Pinoresinol/lariciresinol reductase (PLR), an NADPH-dependent reductase, converts pinoresinol to lariciresinol and subsequently to secoisolariciresinol. Here, we present crystal structures of IiPLR1 from Isatis indigotica and pinoresinol reductases (PrRs) AtPrR1 and AtPrR2 from Arabidopsis thaliana, in the apo, substrate-bound and product-bound states. The crystal structures were captured in the apo, substrate-bound and/or product-bound forms. We found that, for all 16 structures we solved, each enzyme adopts a similar head-to-tail dimer conformation, strongly suggesting that each PLR/PrR functions as a homodimer, consistent with the literature that TpPLR1 exists as a dimeric entity in solution. Each structure contains a head-to-tail homodimer, and the catalytic pocket comprises structural elements from both monomers. β4 loop covers the top of the pocket, and residue 98 from the loop governs catalytic specificity.

Known exceptions are Arabidopsis thaliana reductases that have substrate preference for pinoresinol, but only weak (AtPrR1) or no activity (AtPrR2) toward lariciresinol and are thus named pinoresinol reductases (PrRs). Each of IiPLR1_NAP_ + PIN/AtPrR1_NAP_ + PIN/AtPrR2_NAP_ + PIN forms a homodimer, and superimposition of the protomers among the three complexes revealed RMSDs of 0.374, 0.365, and 0.308 Å, respectively. In contrast to IiPLR1_NAP_ + PIN, the β4 loops of AtPrR1_NAP_ + PIN and AtPrR2_NAP_ + PIN can be clearly identified. These well-defined loops twist as an “8” shape and cover both the NADP+-binding and substrate-binding grooves. Within the twisted loop, His93 and His97 “grasp” helices α5 and α10, while Val92 and Phe94 interact directly with (+)-pinoresinol; Arg95 strongly interacts with NADP+ as well as each of the GXXGXXG motif and α2-helix from neighboring protomer of the dimer. Similar conformational changes of β2 loop and α10-helix can be seen by comparing the structure of AtPrR1_NAP_ + PIN with that of AtPrR1_NAP and the structure of AtPrR2_NAP_ + PIN with that of AtPrR2_apo. Although Val46 is unchanged in AtPrR2, the α2-helix and β2 loop from the neighboring protomer move closer to the substrate upon its entry at the catalytic site, further condensing the pocket. The relative movement of dimers between AtPrR2 and IiPLR1 (as suggested by the ~9° shift shown in Fig. 3c) could be induced by different dimer orientations. Two molecules of the dimer exhibit relative torsion in AtPrR2, and consequently, Val46 is forced deeper into the substrate-binding pocket compared with what occurs in IiPLR1. Therefore, the entrance and orientation of the substrate in AtPrR1/2 is more tightly controlled than in IiPLR1.

> MKETNFGEKTRVLVVGGTGSLGRRIVSACLAEGHETYVLQRPEIGVDIEKVQLLLSFKRLGAHLVEGSFSDHQSLVSAVKQVDVVVSAMSGVHFRTHNIPVQLKLVAAIKEAGNVKRFLPSEFGMDPSRMGHAMPPGSETFDQKMEIRNAIKAAGISHTYLVGACFAAYFGGNLSQMGTLFPPKNKVDIYGDGNVKVVFVDEDDMAKYTAKTLNDPRTLNKTVYVRPTDNILTQMELVQIWEKLTEKELEKTYVSGNDFLADIEDKEISHQAGLGHFYHIYYEGCLTDHEVGDDEEATKLYPDVKYKRMDEYLKIFV>GSHMENMGTRVIEPLIMGRVVGDVLDFFTPTTKMNVSYNKKQVSNGHELFPSSVSSKPRVEIHGGDLRSFFTLVMIDPDVPGPSDPFLKEHLHWIVTNIPGTTDATFGKEVVSYELPRPSIGIHRFVFVLFRQKQRRVIFPNIPSRDHFNTRK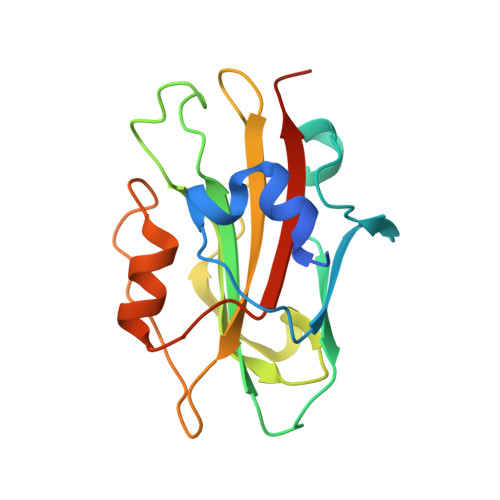FAVEYDLGLPVAAVFFNAQRETAARKR[2x]>MALVEDNNAVAVSFSEEQEALVLKSWAILKKDSANIALRFFLKIFEVAPSASQMFSFLRNSDVPLEKNPKLKTHAMSVFVMTCEAAAQLRKAGKVTVRDTTLKRLGATHLKYGVGDAHFEVVKFALLDTIKEEVPADMWSPAMKSAWSEAYDHLVAAIKQEMK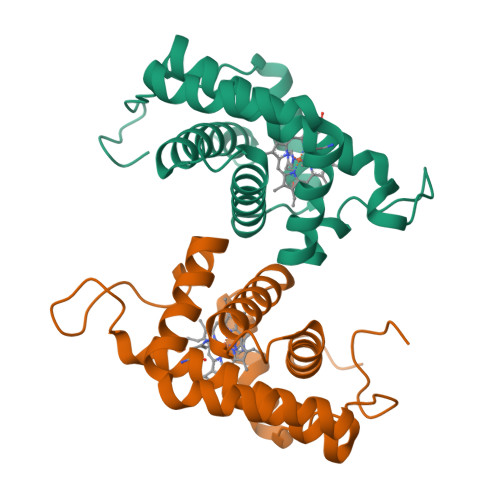PAE[2x]>GPAMQDTVTKKGTGNFTAHGDIIHKTYKEEFPNEG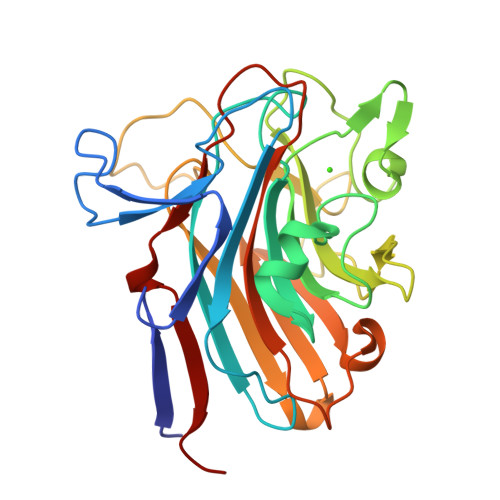TLTAFNTNFNPNTGTKGALEYNDKIDFNKDFTITVPVANNNQGNTTGADGWGFMFTQGNGQDFLNQGGILRDKGMANASGFKIDTAYNNVNGKVDKLDADKTNNLSQIGAAKVGYGTFVKNGADGVTNQVGQNALNTKDKPVNKIIYADNTTNHLDGQFHGQRLNDVVLNYDAATSTITATYAGKTWKATTDDLGIDKSQKYNFLITSSHMQNRYSNGIMRTNLEGVTITTPQAD[2x]>[2x]NAKRIEGLDSNVWVEFTKLAADPSVVNLGQGFPDISPPSYVKEELSKAAFIDNMNQYTRGFGHPALVKALSCLYGKIYQRQIDPNEEILVAVGAYGSLFNSIQGLVDPGDEVI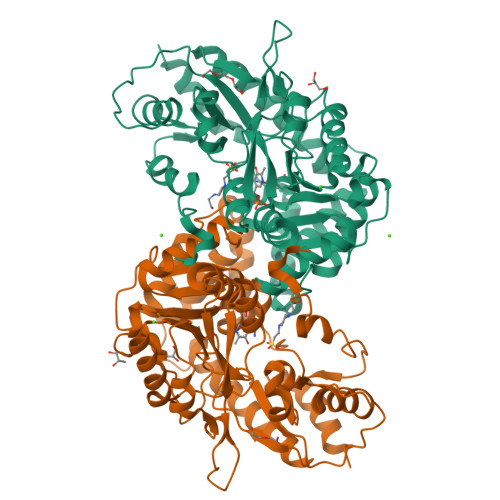IMVPFYDCYEPMVRMAGAVPVFIPLRSKPTDGMKWTSSDWTFDPRELESKFSSKTKAIILNTPHNPLGKVYTRQELQVIADLCVKHDTLCISDEVYEWLVYTGHTHVKIATLPGMWERTITIGSAGKTFSVTGWKLGWSIGPAHLIKHLQTVQQNSFYTCATPLQAALAEAFWIDIKRMDDPECYFNSLPKELEVKRDRMVRLLNSVGLKPIVPDGGYFIIADVSSLGADLSDMNSDEPYDYKFVKWMTKHKKLTAIPVSAFCDSKSKPHFEKLVRFCFIKKDSTLDAAEEIFRAWN> GSSETSVNRGPEKIRPECFELLRVL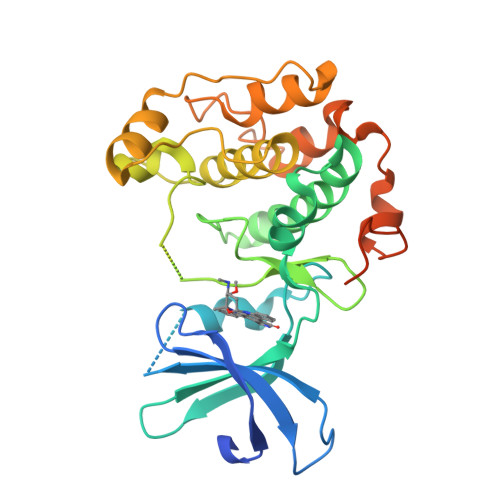GKGGYGKVFQVRKVTGANTGKIFAMKVLKKAMIVRNAKDTAHTKAERNILEEVKHPFIVDLIYAFQTGGKLYLILEYLSGGELFMQLEREGIFMEDTACFYLAEISMALGHLHQKGIIYRDLKPENIMLNHQGHVKLTDFGLCKESIHDGTVTHTFCGTIEYMAPEILMRSGHNRAVDWWSLGALMYDMLTGAPPFTGENRKKTIDKILKCKLNLPPYLTQEARDLLKKLLKRNAASRLGAGPGDAGEVQAHPFFRHINWEELLARKVEPPFKPLLQSEEDVSQFDSKFTRQTPVDSPDDST>MQGSVTEFLKPRLVDIEQVSSTHAKVTLEPLERGFGHTLGNALRRILLSSMPGCAVTEVEIDGVLHEYSTKEGVQEDILEILLNLKGLAVRVQGKDEVILTLNKSGIGPVTAADITHDGDVEIVKPQHVICHLTDENASISMRIKVQRGRGYVPASTRIHSEEDERPIGRLLVDACYSPVERIAYNVEAARVEQRTDLDKLVIEMETNGTIDPEEAIRRAATILAEQLEAFVDLRDVRQPEVKEEKPEFDPILLRPVDDLELTVRSANCLKAEAIHYIGDLVQRTEVELLKTPNLGKKSLTEIKDVLASRGLSLGMRLENWPPASIADEKL[2x];> MEFVYSYTEKKRIRKDFGKRPQVLDVPYLLSIQLDSFQKFIEQDPEGQYGLEAAFRSVFPIQSYSGNSELQYVSYRLGEPVFDVQECQIRGVTYSAPLRVKLRLVIYEREAPEGTVKDIKEQEVYMGEIPLMTDNGTFVINGTERVIVSQLHRSPGVFFDSDKGKTHSSGKVLYNARIIPYRGSWLDFEFDPKDNLFVRIDRRRKLPATIILRALNYTTEQILDLFFEKVIFEIRDNKLQMELVPERLRGETASFDIEANGKVYVEKGRRITARHIRQLEKDDVKLIEVPVEYIAGKVVAKDYIDESTGELICAANMELSLDLLAKLSQSGHKRIETLFTNDLDHGPYISETLRVDPTNDRLSALVEIYRMMRPGEPPTREAAESLFENLFFSEDRYDLSAVGRMKFNRSLLREEIEGSGILSKDDIIDVMKKLIDIRNGKGEVDDIDHLGNRRIRSVGEMAENQFRVGLVRVERAVKERLSLGDLDTLMPQDMINAKPISAAVKEFFGSSQLSQFMDQNNPLSEITHKRRISALGPGGLTRERAGFEVRDVHPTHYGRVCPIETPEGPNIGLINSLSVYAQTNEYGFLETPYRKVTDGVVTDEIHYLSAIEEGNYVIAQANSNLDEEGHFVEDLVTCRSKGESSLFSRDQVDYMDVSTQQVVSVGASLIPFLEHDDANRALMGANMQRQAVPTLRADKPLVGTGMERAVAVDSGVTAVAKRGGVVQYVDASRIVIKVNEDEMYPGEAGIDIYNLTKYTRSNQNTCINQMPCVSLGEPVERGDVLADGPSTDLGELALGQNMRVAFMPWNGYNFEDSILVSERVVQEDRFTTIHIQELACVSRDTKLGPEEITADIPNVGEAALSKLDESGIVYIGAEVTGGDILVGKVTPKGETQLTPEEKLLRAIFGEKASDVKDSSLRVPNGVSGTVIDVQVFTRDGVEKDKRALEIEEMQLKQAKKDLSEELQILEAGLFSRIRAVLVAGGVEAEKLDKLPRDRWLELGLTDEEKQNQLEQLAEQYDELKHEFEKKLEAKRRKITQGDDLAPGVLKIVKVYLAVKRRIQPGDKMAGRHGNKGVISKINPIEDMPYDENGTPVDIVLNPLGVPSRMNIGQILETHLGMAAKGIGDKINAMLKQQQEVAKLREFIQRAYDLGADVRQKVDLSTFSDEEVMRLAENLRKGMPIATPVFDGAKEAEIKELLKLGDLPTSGQIRLYDGRTGEQFERPVTVGYMYMLKLNHLVDDKMHARSTGSYSLVTQQPLGGKAQFGGQRFGEMEVWALEAYGAAYTLQEMLTVKSDDVNGRTKMYKNIVDGNHQMEPGMPESFNVLLKEIRSLGINIELEDESR;> MTDKMQSLALAPVGNLDSYIRAANAWPMLSADEERALAEKLHYHGDLEAAKTLILSHLRFVVHIARNYAGYGLPQADLIQEGNIGLMKAVRRFNPEVGVRLVSFAVHWIKAEIHEYVLRNWRIVKVATTKAQRKLFFNLRKTKQRLGWFNQDEVEMVARELGVTSKDVREMESRMAAQDMTFDLSSDDDSDSQPMAPVLYLQDKSSNFADGIEDDNWEEQAANRLTDAMQGLDERSQDIIRARWLDEDNKSTLQELADRYGVSAERVRQLEKNAMKKLRAAIEA;> MTSKDLLKFLKAQTKTEEFDAIKIALASPDMIRSWSFGEVKKPETINYRTFKPERDGLFCARIFGPVKDYECLCGKYKRLKHRGVICEKCGVEVTQTKVRRERMGHIELASPTAHIWFLKSLPSRIGLLLDMPLRDIERVLYFESYVVIEGGMTNLERQQILTEEQYLDALEEFGDEFDAKMGAEAIQALLKSMDLEQECEQLREELNETNSETKRKKLTKRIKLLEAFVQSGNKPEWMILTVLPVLPPDLRPLVPLDGGRFATSDLNDLYRRVINRNNRLKRLLDLAAPDIIVRNEKRMLQEAVDALLDNGRRGRAITGSNKRPLKSLADMIKGKQGRFRQNLLGKRVDYSGRSVITVGPYLRLHQCGLPKKMALELFKPFIYGKLELRGLATTIKAAKKMVEREEAVVWDILDEVIREHPVLLNRAPTLHRLGIQAFEPVLIEGKAIQLHPLVCAAYNADFDGDQMAVHVPLTLEAQLEARALMMSTNNILSPANGEPIIVPSQDVVLGLYYMTRDCVNAKGEGMVLTGPKEAERLYRSGLASLHARVKVRITEYEKDANGELVAKTSLKDTTVGRAILWMIVPKGLPYSIVNQALGKKAISKMLNTCYRILGLKPTVIFADQIMYTGFAYAARSGASVGIDDMVIPEKKHEIISEAEAEVAEIQEQFQSGLVTAGERYNKVIDIWAAANDRVSKAMMDNLQTETVINRDGQEEKQVSFNSIYMMADSGARGSAAQIRQLAGMRGLMAKPDGSIIETPITANFREGLNVLQYFISTHGARKGLADTALKTANSGYLTRRLVDVAQDLVVTEDDCGTHEGIMMTPVIEGGDVKEPLRDRVLGRVTAEDVLKPGTADILVPRNTLLHEQWCDLLEENSVDAVKVRSVVSCDTDFGVCAHCYGRDLARGHIINKGEAIGVIAAQSIGEPGTQLTMRTFHIGGAASRAAAESSIQVKNKGSIKLSNVKSVVNSSGKLVITSRNTELKLIDEFGRTKESYKVPYGAVLAKGDGEQVAGGETVANWDPHTMPVITEVSGFVRFTDMIDGQTITRQTDELTGLSSLVVLDSAERTAGGKDLRPALKIVDAQGNDVLIPGTDMPAQYFLPGKAIVQLEDGVQISSGDTLARIPQESGGTKDITGGLPRVADLFEARRPKEPAILAEISGIVSFGKETKGKRRLVITPVDGSDPYEEMIPKWRQLNVFEGERVERGDVISDGPEAPHDILRLRGVHAVTRYIVNEVQDVYRLQGVKINDKHIEVIVRQMLRKATIVNAGSSDFLEGEQVEYSRVKIANRELEANGKVGATYSRDLLGITKASLATESFISAASFQETTRVLTEAAVAGKRDELRGLKENVIVGRLIPAGTGYAYHQDRMRRRAAGEAPAAPQVTAEDASASLAELLNAGLGGSDNELEHHHHHHHHHHHHGT

During bacterial transcription initiation, σ factors associate with the RNAP core enzyme, guide the transcription machinery to promoter regions of genes, and engage double-strand promoter DNA. Primary σ factor (group 1) is responsible for transcription of housekeeping genes, while alternative σ factors (group 2, group 3, and group 4) control transcription of genes during adaptation to certain intracellular and environmental signals. The group 3 σ factor, σ32, plays a pivotal role in the heat shock response (HSR) required by E. coli to sustain protein homeostasis and cope with heat and other stresses. σ32 synthesis is modulated by the secondary structure of the 5′ region of σ32 mRNA, which serves as a “thermometer”, responding to temperature changes. When the temperature for growing E. coli cells suddenly increases, σ32 is rapidly synthesized (induction phase) and then directs RNA polymerase to promote transcription of a set of HSR genes to respond to environmental temperature changes.

To determine the structure of E. coli σ32-RPo, we reconstituted the complex with the E. coli RNAP core enzyme, σ32, and a nucleic acid scaffold. The nucleic acid scaffold (−39 to +15; +1 as transcription start site) is composed of a 28-bp upstream double-stranded DNA (dsDNA) with consensus sequences of the −35 element, a 13-bp transcription bubble (complementary sequences on both strands), and a 13-bp downstream dsDNA. We obtained a cryo-EM map at 3.0 Å for the E. coli σ32-RPo complex with local resolution at the active-center cleft of RNAP around 2.49 Å. Similar to other σ factors, the RNAP clamp in the structure of σ32-RPo remains in a closed conformation. The omega subunit is absent from the solved structure, probably due to low binding affinity. The σ2 domain attaches to the clamp helices of the β′ subunit of RNAP via a polar surface. The σ4 domain of σ32 uses a distinct hydrophobic surface to bind the βFTH of RNAP. In the structure, σ4 adopts a helix-turn-helix fold, inserts into the major groove of dsDNA around the −35 element, and potentially makes base-specific polar interactions with nucleotides. K130 of σ32 makes a H-bond with N7 atoms of G−15 on the template DNA strand, which together with G−14 were identified to be the “extend −10” element. Specifically, H107 blocks the path upstream dsDNA and serves as a wedge to disrupt base stacking between positions A−11 and C−12.> MSSLSRELVFLILQFLDEEKFKETVHKLEQESGFFFNMKYFEEKVHAGEWDEVEKYLSGFTKVDDNRYSMKIFFEIRKQKYLEALDRHDRAKAVDILVKDLKVFSTFNEEAYKEITQLL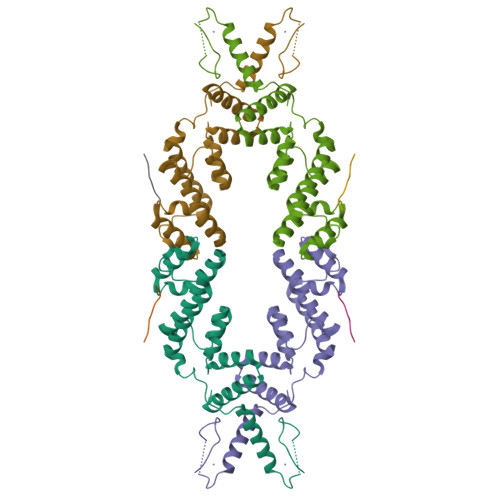TLENFRENEQASKYGDTKSARSIMLIELKKLIEANPLFREKLVFPTLKASRLRTLINQSLNWQHQLCKNPRPNPDIKTLFTDHTCTPPNG;> DNLIYLDLNLQDWDD>MAVLKIISWNVNGLRAVHRKGFLKWFMEEKPDILC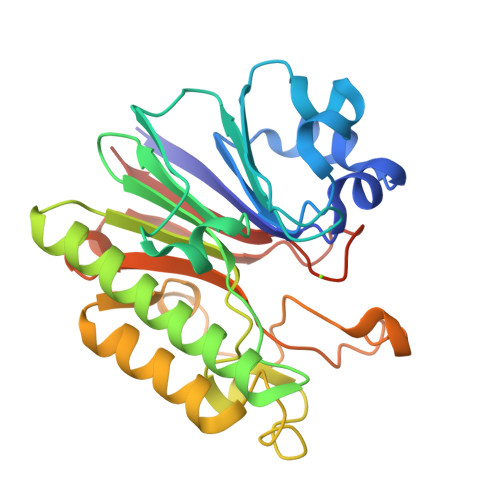LQEIKAAPEQLPRKLRHVEGYRSFFTPAERKGYSGVAMYTKVPPSSLREGFGVERFDTEGRIQIADFDDFLLYNIYFPNGKMSEERLKYKLEFYDAFLEDVNRERDSGRNVIICGDFNTAHREIDLARPKENSNVSGFLPVERAWIDKFIENGYVDTFRMFNSDPGQYTWWSYRTRARERNVGWRLDYFFVNEEFKGKVKRSWILSDVMGSDHCPIGLEIELLEHHHHHH[2x]>[10x]GSHMEEVSEYCSHMIGSGHLQSLQRLIDSQMETSCQITFEFVDQEQLKDPVCYLKKAFLLVQDIMEDTMRFRDNTPNAIAIVQLQE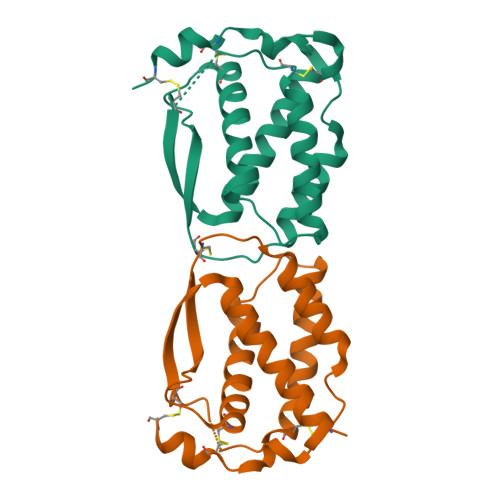LSLRLKSCFTKDYEEHDKACVRTFYETPLQLLEKVKNVFNETKNLLDKDWNIFSKNCNNSFAECSSQ> MLSISAVQRRYRLFHPVHQTVPFHFNPVQSIFPLIYENNLLAKPRLSWKDYEGRKEFDADHPLPVVGTRLNERTTTHKWSHWDQYINPQITQSWMYLTQTPEYVGPRSGHNVIKMGWMKIGGSWKYSRSYNDARRGFAKGQWQERKMTPRFMLAPRVSAGGPRNRYEGKASFSRLSLSKLLWAVDTGRLNPNETITLYHLRNAKVIADREVVWPGMVLLAGNVERVPYPLHIELQNASAKAIQLLEEAGGSFTNVYMSHEGLYQELHPEEFPTFMEQELPERKGL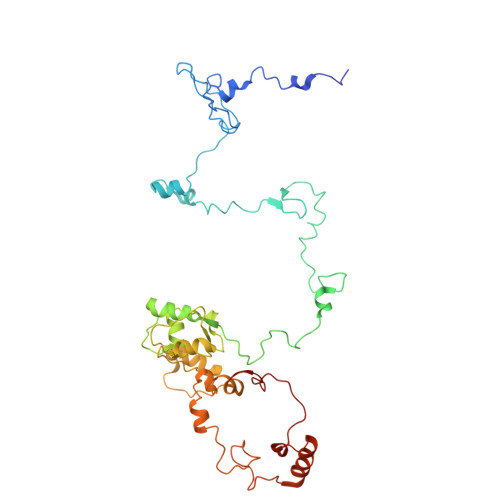ENFATNSRKRGWLAQWYEDESRYAHPGAGRRTAHYIRPPTDRDFPATIEEYELAKHHQKWHLNQPGSATVLPWHSLNTADMARRSAGRL>MQYKKIITSESVGAGHPDKICDQISDAILDECLSQDQNSRVACEVLACNRLIVIAGEITTHAYVDVVKTAWEIIKPLGYDENDFTIISNVNKQSVDIAQSVDKTNKNLIGAGDQGIVFGYACDETPQYMPLTSVLAHELLKEIERQRRSKEFIKIQADMKSQVSIDYSNSTPLIETMLVSIQHDEDYDVE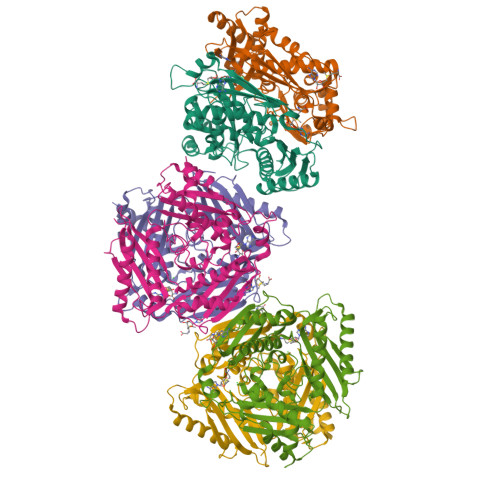YFNKKVSAIMEQIAKKYNLNTNFKKIINSSGRFVIGGPIGDTGLTGRKIIVDTYGGVGHHGGGAFSGKDPTKVDRSASYFARWIAKNVVAAKLAKQCEIQLAFAIGQPQPVAMYVNTFNTNLIDETKIFEAIKKSFNFDIKTFINDLNLWTTKYLPVATYGHFGRDDLDLSWEKLNKVEDLIKNSKHHHHHH[6x]2-azanyl-8-[(2-fluorophenyl)methylsulfanyl]-1,9-dihydropurin-6-one | 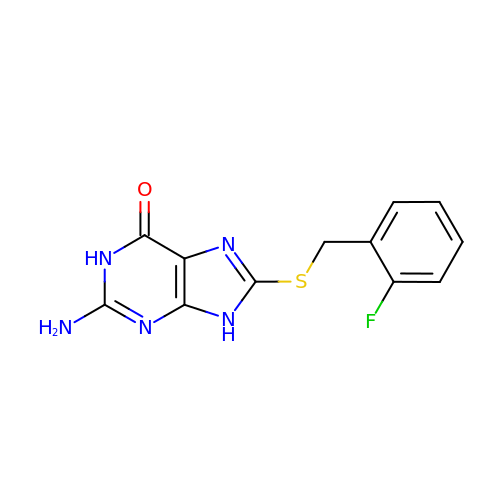C12 H10 F N5 O S | DBXBVKPIQPXRBY-UHFFFAOYSA-N> CKGADGAHGVUGCPGTAGAAGSVGGPGCDGGHGGNGGNGNPGCAGGVGGAGGASG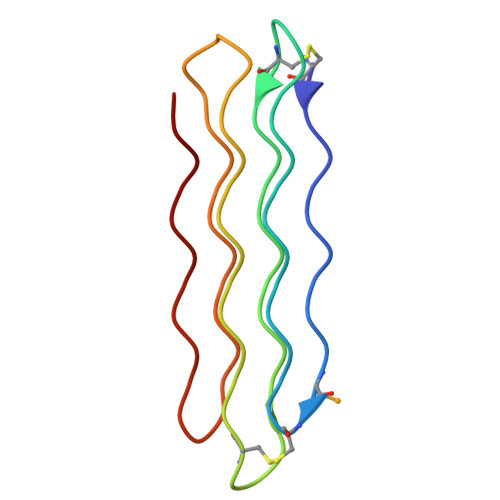GTGVGGRGGKGGSGTPKGADGAPGAP> VQYLNQELVVSGKIDFENAEQQYQAGLAIIKKQTSFPLIVDLKQLEH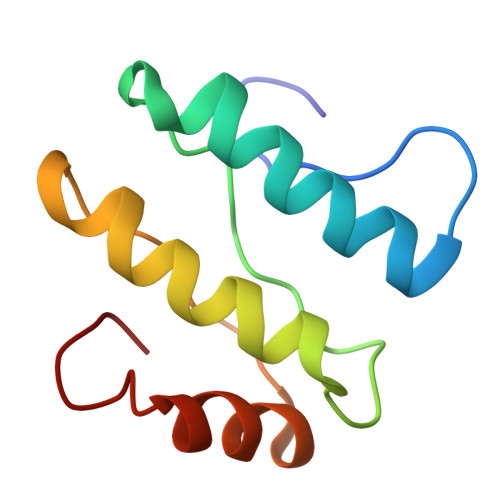GNTLALAVLVQWLRQTPQKSGLHFKNVPEKMLKIIQACHLQEDLHL>[2x]TSALIERIDAIIVDLPTIRPHKLAMHTMQQQTLVVLRVRCSDGVEGIGEATTIGGLAYGYESPEGIKANIDAHLAPALIGLAADNINAAMLKLD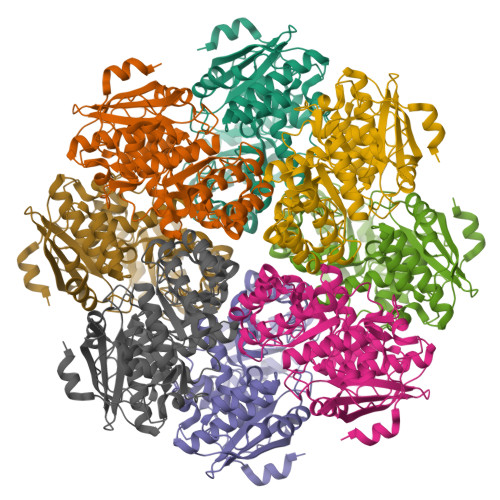ALAKGNTFAKSGIESALLDAQGKRLGLPVSELLGGRVRDSLEVAWTLASGDTARDIAEARHMLEIRRHRVFKLKIGANPVEQNLKHVVTIKRELGDSASVRVDVNQYWDESQAIRACQVLGDNGIDLIEQPISRINRGGQVRLNQRTPAPIMADESIESVEDAFSLAADGAASIFALKIAKNGGPRAVLRTAQIAEAAGIGLYGGTMLEGSIGTLASAHAFLTLRQLTWGTELFGPLLLTEEIVNEPPQYRDFQLHIPRTPGLGLTLDEARLARFARR Haloalkane dehalogenases (HLDs; EC 3.8.1.5) form a family of enzymes that catalyze hydrolytic cleavage of carbon-halogen bond in a wide range of halogenated aliphatic hydrocarbons and their derivatives via SN2 nucleophilic substitution followed by the addition of water, and releasing a halide ion, one proton, and the corresponding alcohol as reaction products. The structure of HLDs is composed of a conserved main (or core) domain, consisting of eight-stranded β-sheet and six α-helices, and a versatile cap domain formed mostly by α-helices. In the present paper, we describe the biochemical and structural characterization of a new HLD from psychrophilic bacterium Marinobacter sp. ELB17, paradoxically possessing the highest thermostability among all biochemically characterized wild type enzymes from HLD-II subfamily. Crystallographic analysis revealed three unique features of DmxA that can contribute to its unusual thermostability: (i) a unique composition of catalytic pentad, possibly lacking one out of the two halide-stabilizing residues; (ii) enzyme dimerization due to a disulfide bridge; and (iii) unusually narrow tunnels connecting the buried enzyme active site with the surrounding solvent.

The crystal structure of DmxA wt was determined by molecular replacement and refined using diffraction data to 1.45 Å. DmxA wt was crystallized in a primitive orthorhombic crystal form, encompassing two protein molecules in the asymmetric unit. The two molecules in the asymmetric unit represent the dimeric form of the enzyme, which was also observed in solution. DmxA wt contains four out of the five canonical catalytic residues in the active site: the nucleophile D105, the catalytic acid E129 and the catalytic base H273, forming catalytic triad, and one halide-stabilizing residue W106. The second halide-stabilizing residue, which is asparagine in HLD-II subfamily, is Q40 in DmxA wt. During the refinement of DmxA wt crystal structure, the electron density present in the vicinity of the active site was interpreted as a water molecule and an acetate ion with an occupancy of 1.0 for both molecules present in the asymmetric unit. The water molecule (HOH511) is situated in a canonical halide-binding pocket of the enzyme and interacts with the nitrogen atom of one halide-stabilizing residue W106 Nε1 at a distance of 2.94 Å. The side chain of Q40 faces away from the halide-binding site and makes polar interactions with the side chain hydroxyl of Y68 and the main chain carbonyl of L203. This suggests that Q40 residue cannot be involved in the stabilization of the substrate nor releasing halide anion in DmxA wt active site. Interactions in the dimeric interface are mediated by 3 salt bridges, 10 hydrogen bonds and, interestingly, an intermolecular disulfide bond formed by cysteine 294 residues from each monomer.

>MTTQKPADFPYPSHFADVLGSRMHYVEHGNGDPLLFLHGQPTWSYLWRKVLPELEGKGRLIAVDLIGYGMSDKPDIPYDIDDHIRYLDGFIEALGLDRITIVCHDWGSFFGFHYAHRHPERIKGLAFMEAMLNPIPGYDAFDPQTRAFFQTLRSSQANAERMMMDENQFVENILPAMICRPLERQELDAYRAPWTDRQSRRILCTFPQNLCIGKEPASVYRMQTAYIEWLGQTDLPKLLIHAEPGFLIPAPAVDQYRQQLPNLETAFVGSGLHYIQEDQPQKIGQAIAQWMDRCGLHHHHHH[2x]>SNAQLTF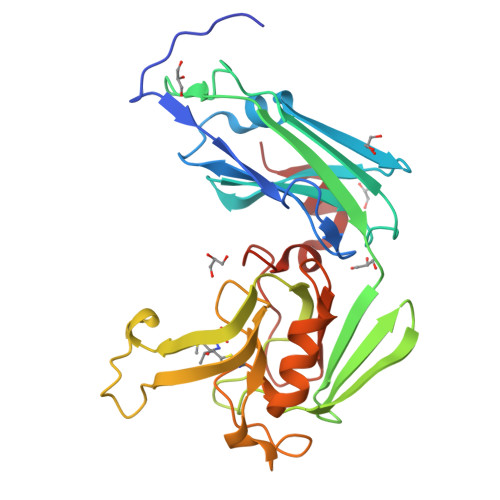QTSSPAHLTMPYVMPGDGEVVGVGEPVAIRFDENIADRGAAEKAIKITTNPPVEGAFYWLNNREVRWRPEHFWKPGTAVDVAVNTYGVDLGEGMFGEDNVQTHFTIGDEVIATADDNTKILTVRVNGEVVKSMPTSMGKDSTPTANGIYIVGSRYKHIIMDSSTYGVPVNSPNGYRTDVDWATQISYSGVFVHSAPWSVGAQGHTNTSHGCLNVSPSNAQWFYDHVKRGDIVEVVNTVGGTLPGIDGLGDWNIPWDQWRAGNAKA[6x]>GHMGQKASQQLALKDSKEVPVVCEVVSEAIVHAAQKLKEYLGFEYPPSKLCPAANTLNEIFLIHFITFCQEKGVDEWLTTTKMTKHQAFLFGADWIWTFWGSDKQIKLQLAVQTLQMSSPPPVESKPCDLSNPESRVEESSWKKSRFDKLEEFCNLIGEDCLGLFIIFGMPGKPKDIRGVVLDSVKSQMVRSHLPGGKAVAQFVLETEDCVFIKELLRNCLSKKDGLREVGKVYISIL[2x];>GHMASVTDGKTGVKDASDQNFDYMFKLLIIGNSSVGKTSFLFRYADDTFTPAFVSTVGIDFKVKTVYRHEKRVKLQIWDTAGQERYRTITTAYYRGAMGFILMYDITNEESFNAVQDWATQIKTYSWDNAQVILVGNKCDMEEERVVPTEKGQLLAEQLGFDFFEASAKENISVRQAFERLVDAICDKMSDSLDTDPSMLGSSKNTRLSDTPPLLQQNCSC[2x]

One such Rab15 effector is Rep15, which is known to have a role in receptor recycling from the endocytic recycling compartment but otherwise remains poorly characterized. Biochemical validation of the interactions is presented and crystal structures of the Rep15:Rab3B and Rep15:Rab3C complexes provide additional mechanistic insight. We find that Rep15 adopts a globular structure that is distinct from other reported Rab15, Rab3 and Rab34 effectors. Detailed biochemical studies reveal that Rep15 is selective for Rab15, Rab3 paralogs and Rab34 and does not bind to other evolutionarily similar Rab GTPases.

All obtained complexes were used to perform the crystallization screen and finally, we obtained crystals for Rep15:Rab3CGppNHp_Q222H_10-227 (bovine), Rep15:Rab3BGppNHp and Rep15_ΔN1:Rab3BQ81L_18-190 complexes. Subsequently, we also obtained Rep15:Rab3BGppNHp and Rep15 ΔN1:Rab3BQ81L_18-190 complex crystals, which diffracted to a resolution 2.75 Å and 2.8 Å, respectively and crystallized in space group C2 and P21 respectively. We solved the Rep15:Rab3B complex structure using Rep15:Rab3C (bovine) as a MR model and Rep15 ΔN1:Rab3BQ81L_18-190 complex structure using Rep15:Rab3BGppNHp complex structure as a MR model. The asymmetric unit contained two copies of the complex. Both copies share nearly the same overall architecture, as indicated by an RMSD of 0.124 Å for Rep15:Rab3BGppNHp complex and and an RMSD of 0.109 Å for the both copies of Rep15 ΔN1:Rab3BQ81L_18-190 complex. Structurally-based sequence alignment of Rab3A and Rab3C shows that apart from the switch I, interswitch and switch II residues, three RabCDRs of Rab3A are involved in making contacts with the Rabphilin-3A, whereas in the case of the Rep15:Rab3 complex structures, RabCDRs are not part of the binding interface.>MGEIRPTIGQQMETGDQRFGDLVFRQLAPNVWQHTSYLDMPGFGAVASNGLIVRDGGRVLVVDTAWTDDQTAQILNWIKQEINLPVALAVVTHAHQDKMGGMDALHAAGIATYANALSNQLAPQEGMVAAQHSLTFAANGWVEPATAPNFGPLKVFYPGPGHTSDNITVGIDGTDIAFGGCLIKDSKAKSLGNLGDADTEHYAASARAFGAAFPKASMIVMSHSAPDSRA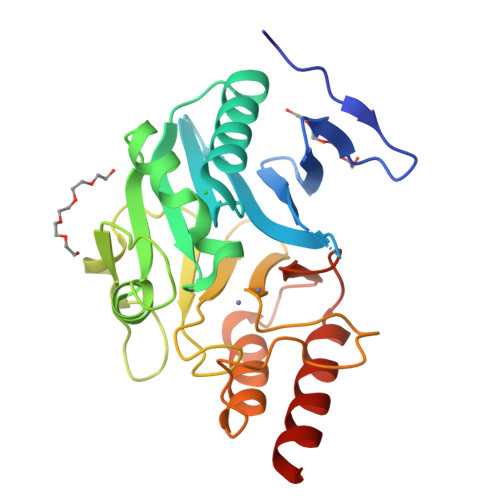AITHTARMADKLRLEHHHHHH[2x]> GSQQFPQFHVKSGLQIKKNAIIDD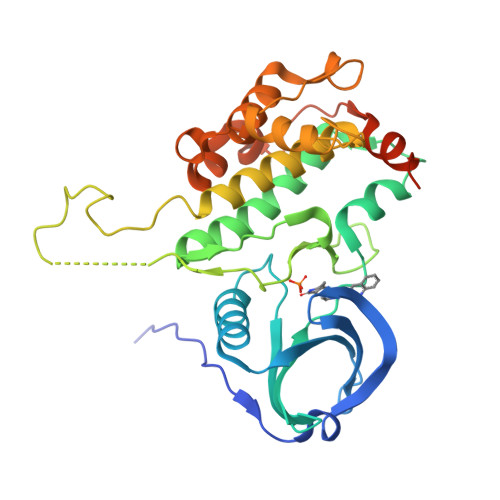YKVTSQVLGLGINGKVLQIFNKRTQEKFALKMLQDCPKARREVELHWRASQCPHIVRIVDVYENLYAGRKCLLIVMECLDGGELFSRIQDRGDQAFTEREASEIMKSIGEAIQYLHSINIAHRDVKPENLLYTSKRPNAILKLTDFGFAKETTSHNSLTTPCYTPYYVAPEVLGPEKYDKSCDMWSLGVIMYILLCGYPPFYSNHGLAISPGMKTRIRMGQYEFPNPEWSEVSEEVKMLIRNLLKTEPTQRMTITEFMNHPWIMQSTKVPQTPLHTSRVLKEDKERWEDVKEEMTSALATMR> SMQSSKRSSRSVEDDKEGHLVCRIGDWLQERYEIVGNLGEGTFGKVVECLDHARGKSQVALKIIRNVGKYREAARLEINVLKKIKEKDKENKFLCVLMSDWFNFHGHMCIAFELLGKNTFEFLKENNFQPYPLPHVRHMAYQLCHALRFLHENQLTHTDLKPENILFVNSEFETLYNEHKSCEEKSVKNT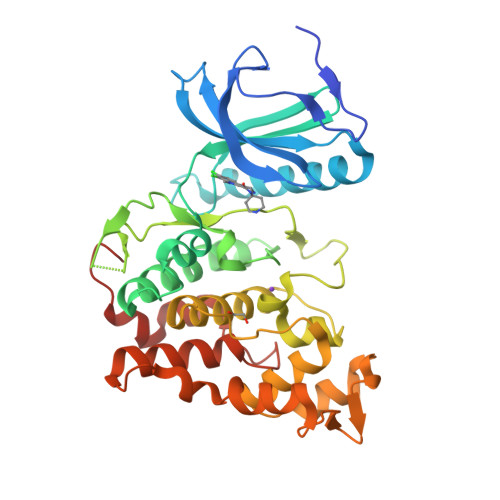SIRVVDFGSATFDHEHHTTIVATRHYRPPEVILELGWAQPCDVWSIGCILFEYYRGFTLFQTHENREHLVMMEKILGPIPSHMIHRTRKQKYFYKGGLVWDENSSDGRYVKENCKPLKSYMLQDSLEHVQLFDLMRRMLEFDPAQRITLAEALLHPFFAGLTPEERSFHT>GCGUACGAAGGAGAGGAGAGGAAGAGGAGAGUACGC[2x];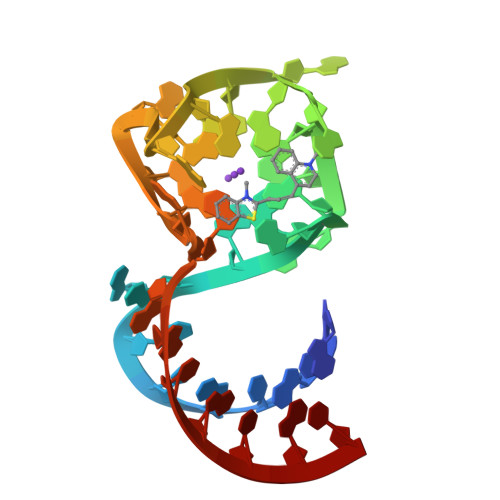> GUACGAAGGAGAGGAGAGGAAGAGGAGAGUAC> 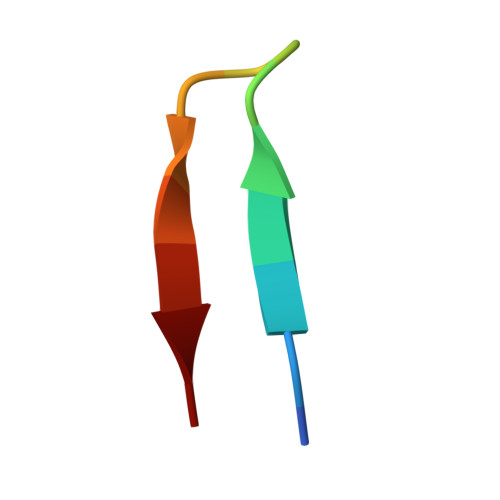HIRGSITQGIPRSY> SGTTNTVAAYNLTWKSTNFKTILEWEPKPVNQVYTVQISTKSGD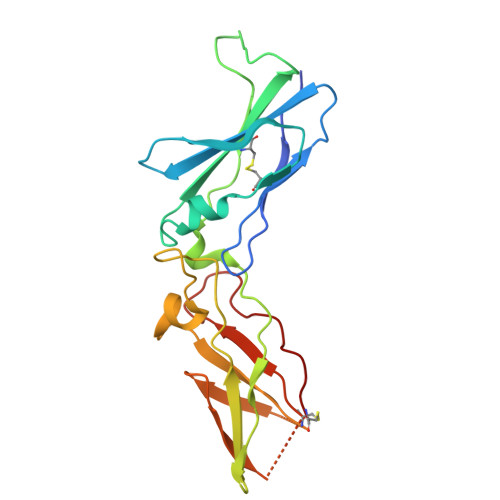WKSKCFYTTDTECDLTDEIVKDVKQTYLARVFSYPAGNVESTGSAGEPLYENSPEFTPYLETNLGQPTIQSFEQVGTKVNVTVEDERTLVRRNNTFLSLRDVFGKDLIYTLYYWKSSSSGKKTAKTNTNEFLIDVDKGENYCFSVQAVIPSRTVNRKSTDSPVEC> MVSDYVP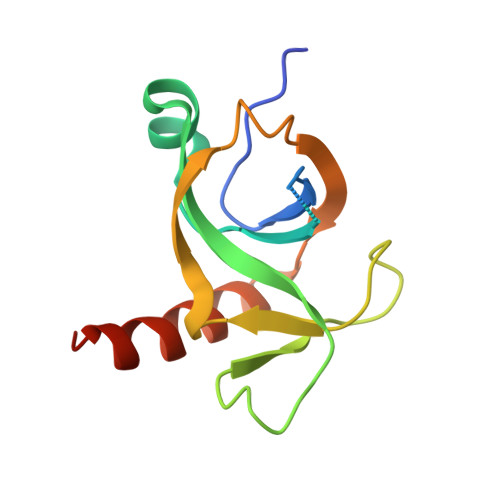DAGHLVWLNFTPQAGHEQGGRRPALVLSPAAYNGVTGLMQACPVTSRAKGYPFEVTLPAHLGVSGVVLADHCRSLDWRSRRAEQLAEAPADVLAEVRGKLGSLLGMSEKA> LLIGFWDCVTCHGSPVDICTAKPRDIPMNPMCIY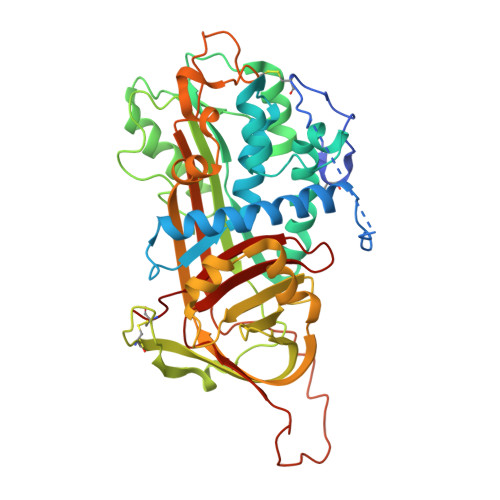RSPEKKATEDEGSEQKIPEATNRRVWELSKANSRFATTFYQHLADSKNDNDNIFLSPLSISTAFAMTKLGACNDTLQQLMEVFKFDTISEKTSDQIHFFFAKLNCRLYRKANKASKLVSANRLFGDKSLTFNETYQDISELVYGAKLQPLDFKENAEQSRAAINKWVSNKTEGRITDVIPSEAINELTVLVLVNTIYFKGLWKSKFSPENTRKELFYKADGESCSASMMYQEGKFRYRRVAEGTQVLELPFKGDDITMVLILPKPEKSLAKVEKELTPEVLQEWLDELEEMMLVVHMPRFRIEDGFSLKEQLQDMGLVDLFSPAASALPGIVAEGRDDLYVSDAFHKAFLEVNEEGSEAAASTAVVIAGRSLNPNRVTFKANRPFLVFIREVPLNTIIFMGRVANPCVK>[2x]RKPIIAGNWKMHKTLAEAVQFVEDVKGHVPPADEVISVVCAPFLFLDRLVQAADGTDLKIGAQTMHFADQGAYTGEVSPVMLKDLGVTYVILGHSERRQMFAETDETVNKKVLAAFTRGLIPIICCGESLEEREAGQTNAVVASQVEKALAGLTPEQVKQAVIAYEPIWAIGTGKSSTPEDANSV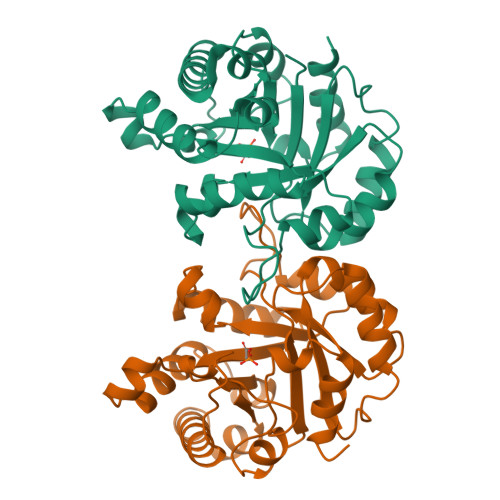CGHIRSVVSRLFGPEAAEAIRIQYGGSVKPDNIRDFLAQQQIDGPLVGGASLEPASFLQLVEAGRHE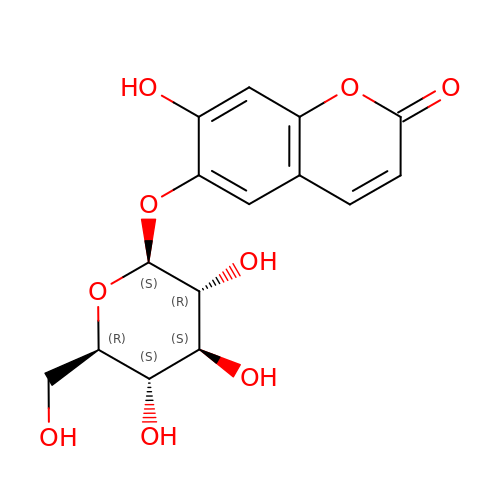6-[(2S,3R,4S,5S,6R)-6-(hydroxymethyl)-3,4,5-tris(oxidanyl)oxan-2-yl]oxy-7-oxidanyl-chromen-2-one | C15 H16 O9 | XHCADAYNFIFUHF-TVKJYDDYSA-N>[2x]MSLSLFVTRLYHAPLSDHGPAIDAEEMESSCYAIAEDDEAGQGWCEENGYPGYTSYASLTDLPWRFPIFADLVKSLDAHVAAFAEDLEFDL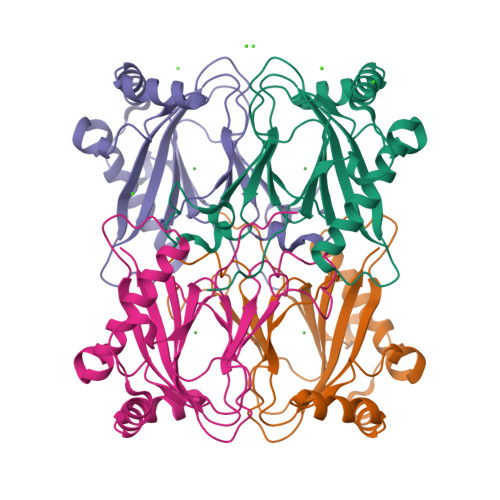DGRALELEDLWINILPEGGSHASHIHPHSVISGTTYVSMPGGTSALKLEDPRHAMMMAAPARRKTARDELRQFIYVTPAVGDVLLWESWLRHEVPMNMSEDDRISVSFNYRWAEGHHHHHH>MKISENWLRTWVNPAIDSDTLSDQLTMLGLEVDELASVAKPFTGVVVGEVLTVEQHPDADRLRVTTVNIGSGEPLQIVCGAPNVRAGMKAPVATIGAVLPGDFKIKK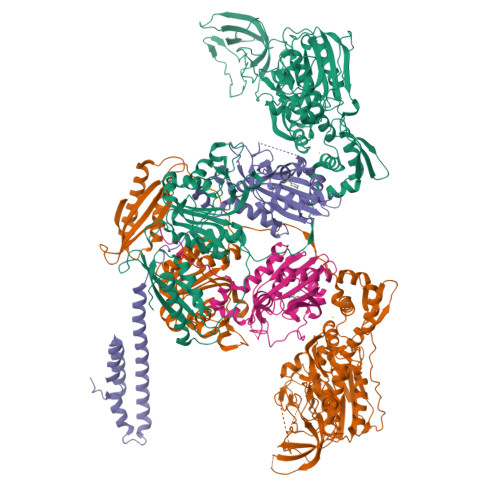GKLRGVESQGMLCGASEIDLEDKIDGLLELPADAPVGVNIREYLKLDDNVIDISITPNRGDCFSIRGIAREVAVINQLQMNEPEIKSVDATITDEKKVVINTDGAPRYLGRVIKNVNVKAATPEWMEQALARSGIRTHSILVDVTNYVLMELGQPMHAFDLAKIEGTVHVRQAKPQEKLQLLNDQEVELQEDVMVIADDQKALAIAGIMGGLASSVTDDTTDIFLESAFFAPLAIAGRARRFGLHTDSSQRYERGVDFELPVIAMNRASQLIQELAGGEFGPITVAEKSDLLPKREAIELKQAQVDQLLGYKVAAEFITDALTRLGCEVTVQANGEWSVVPPSHRYDMAIYQDLIEEVARIDGYDNIQISLPSMDVQLAKYQDRFEIAQLRQTVATLGYQEAISFSFADAKLEKQLNPQVSPLMLANPISSDLAAMRSTLLSSLIPCVQYNLNRQQSRVRFFELGLRFDYQNANSIQDLKQIPTLALVAVGSREPESWHAKPQPMDFFDFKGEVEEILAAGRVKVEYVRSERPWLHPGQSAEILVDGQSIGYLGRLHPSLENELDLSTTWVAELDQAAVLQSYVSNFTELSRFPSVRRDIALLISDNINVRDIQQLIEKTGGELLDSTWLFDVYTGQGVEEGKRSLAFALLWQHPSRTLEDAEIKSGMDNIIQVLENTYQATLRAS[4x];>MRVTMSLEALTTEALAAIAAAQDLVALDQVRVQFTGKKSQLAEQSKALGKMDPEERKVQGAAIHAVRETINNALTERQTALQQAALAQKLASETIDITLPGRGQRIGTVHPVTQVQERICQFFTKAGFTVATGPEVEDDYHNFEALNIPGHHPARAMHDTFYFDANHLLRTHTSGVQIRTMETSQPPIRIVCPGRVYRCDSDQTHSPMFHQIEGLYVAENTSFAELKGLLINLLNEFFEKDLKVRFRPSYFPFTEPSAEVDIMDERGRWLEVLGCGMVHPNVLRAAGIDPDKYKGFAFGLGVERFAMLRYGINDLRMFYQNDVRFLRQFA[4x]(3S)-N-(4-methylbenzyl)-1-{2-[(3,4,5-trimethoxyphenyl)amino]pyrimidin-4-yl}piperidine-3-carboxamide 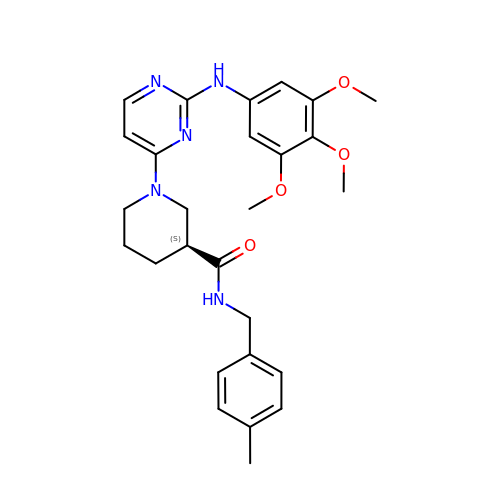| C27 H33 N5 O4 | BAQAWVMHTOQJCI-FQEVSTJZSA-N>MSFTPANRAYPYTRLRRNRRDDFSRRLVRENVLTVDDLILPVFVLDGVNQRESIPSMPGVERLSIDQLLIEAEEWVALGIPALALFPVTPVEKKSLDAAEAYNPEGIAQRATRALRERFPELGIITDVALDPFTTHGQNGILDDDGYVLNDVSIDVLVRQALSHAEAGAQVVAPSDMMDGRIGAIREALESAGHTNVRVMAYSAKYASAYYGPFRDAVGSASNLGKGNKATYQMDPANSDEALHEVAADLAEGADMVMVKPGMPYLDIVRRVKDEF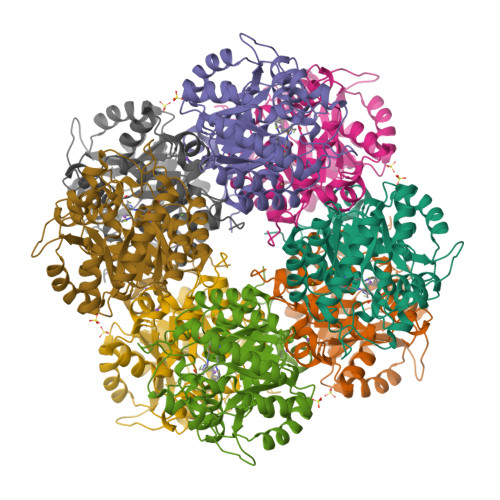RAPTFVYQVSGEYAMHMGAIQNGWLAESVILESLTAFKRAGADGILTYFAKQAAEQLRRGR[2x]>KPPECPDFDPPRQENETWWLCDCFMATCKYNNTVEIVKVECEPPPMPTCSNGLQPVRVEDPDGCCWHWECDCYCTGWGDPHYVTFDGLYYSYQGNCTYVLVEEISPSVDNFGVYIDNYHCDPNDKVSCPRTLIVRHETQEVLIKTVHMMPMQVQVQVNRQAVALPYKKYGLEVYQSGINYVVDIPELGVLVSYNGLSFSVRLPYHRFGNNTKGQCGTCTNTTSDDCILPSGEIVSNCEAAADQWLVNDPSKPHCPHSSSTTKRPAVTVPGGGKTTPHKDCTPSPLCQLIKDSLFAQCHALVPPQHYY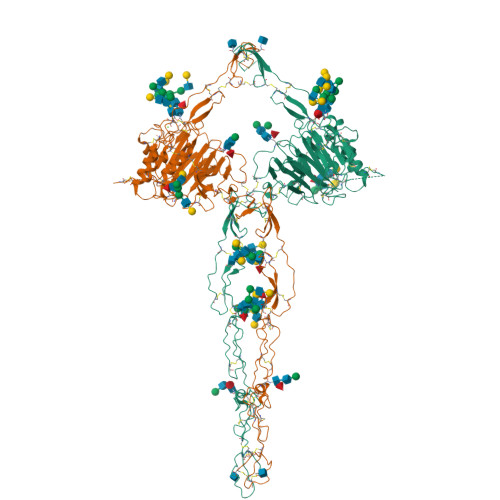DACVFDSCFMPGSSLECASLQAYAALCAQQNICLDWRNHTHGACLVECPSHREYQACGPAEEPTCKSSSSQQNNTVLVEGCFCPEGTMNYAPGFDVCVKTCGCVGPDNVPREFGEHFEFDCKNCVCLEGGSGIICQPKRCSQKPVTHCVEDGTYLATEVNPADTCCNITVCKCNTSLCKEKPSVCPLGFEVKSKMVPGRCCPFYWCESKGVCVHGNAEYQPGSPVYSSKCQDCVCTDKVDNNTLLNVIACTHVPCNTSCSPGFELMEAPGECCKKC[2x]>AHHHHHHMQIIHTIRELRTWRENTGKVAFVPTMGNLHEGHLALVREARKRADNVVVSIFVNRLQFGQGEDFDKYPRTLQQDADKLAAEGVAVVFAPDEKELYPNVEQRYNVEPPHLQNELCGKFRPGHFRGVATVVSKLFNIVLPDVACFGKKDYQQLA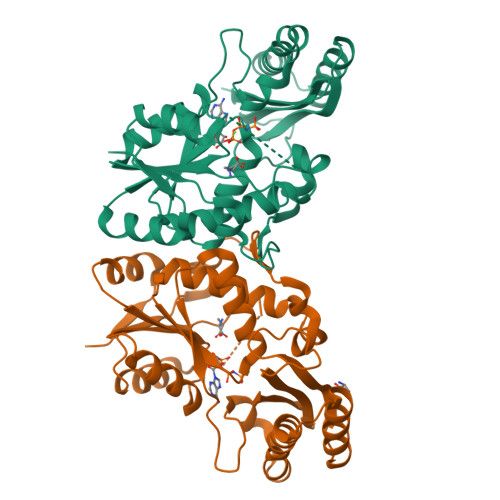VIKGLTEDLNFDIEIVPVDTGRAADGLALSSRNRYLSVGERAEAPRLYRELQAVAESLKQGGLDYAGLERQAADHLTAAGWLVDYVEIRRADTLEMARAGDKKLVVLAAARLGTTRLIDNVEVGLP[2x]>[2x]GMALQLSREQGITARGSAEIVA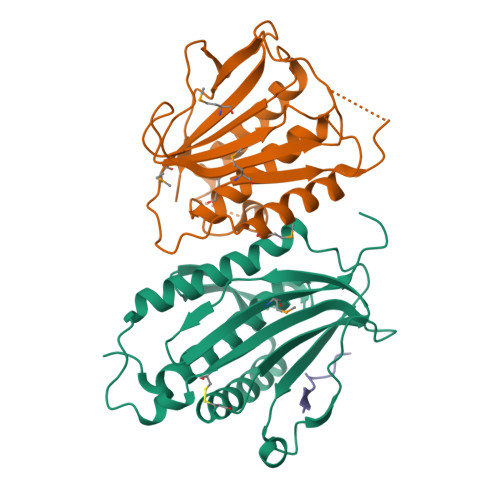EFFSFGINSILYQRGIYPSETFTRVQKYGLTLLVTTDLELIKYLNNVVEQLKDWLYKCSVQKLVVVISNIESGEVLERWQFDIECDKTAKDDSAPREKSQKAIQDEIRSVIRQITATVTFLPLLEVSCSFDLLIYTDKDLVVPEKWEESGPQFITNSEEVRLRSFTTTIHKVNSMVAYKIPVND;>MTSSTQEPLNASEAFCPRDCMVPVVFPGPVSQEGCCQFTCELLKHIMYQRQQLPLPYEQLKHFYRKPSPQAEEMLKKKPRATTEVSSRKCQQALAELESVLSHLEDFFARTLVPRVLILLGGNALSPKEFYELDLSLLAPYSVDQSLSTAACLRRLFRAIFMADAFSELQAPPLMGTVVMAQGHRNCGEDWFRPKLNYRVPSRGHKLTVTLSCGRPSIRTTAWEDYIWFQAPVTFKGFRE[2x];>[2x]SWYSYPPPQRAV N-[(1R)-2-(BENZYLSULFANYL)-1-FORMYLETHYL]-N-(MORPHOLIN-4-YLCARBONYL)-L-PHENYLALANINAMIDE | C24 H29 N3 O4 S | 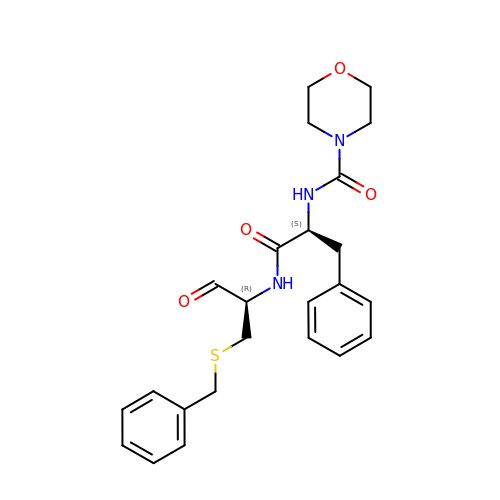MWTQNXVXPLTHJB-YADHBBJMSA-N> LTEDGDSFLHLAIIHEEKALTMEVIRQVKGDLAFLNFQNN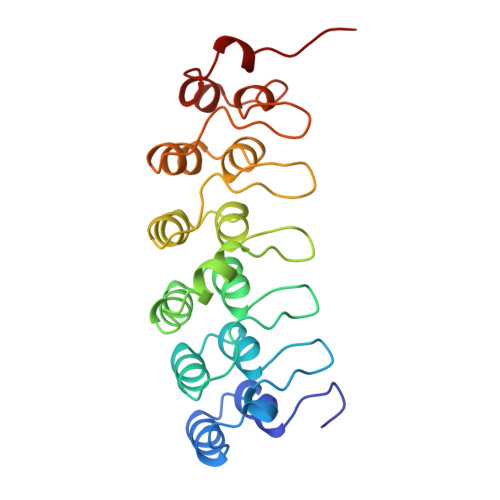LQQTPLHLAVITNQPEIAEALLGAGCDPELRDFRGNTPLHLACEQGCLASVGVLTQSCTTPHLHSILKATNYNGHTCLHLASIHGYLGIVELLVSLGADVNAQEPCNGRTALHLAVDLQNPDLVSLLLKCGADVNRVTYQGYSPYQLTWGRPSTRIQQQLGQLTLENLQMLPE>MKIVDVLCTPGLTGFYFDDQRAIKKGAGHDGFTYTGSTVTEGFTQVRQKGESISVLLVLEDGQVAHGDCAAVQYSGAGGRDPLFLAKDFIPVIEKEIAPKLIGREITNFKPMAEEFDKMTVNGNRLHTAIRYGITQAILDAVAKTRKVTMAEVIRDEYNPGAEINAVPVFAQSGDDRYDNVDKMIIKEADVLPHALINNVEEKLGLKGEKLLEYVKWLRDRIIKLRVREDYAPIFHIDVYGTIGAAFDVDIKAMADYIQTLAEAAKPFHLRIEGPMDVEDRQKQMEAMRDLRAELDGRGVDAELVADEWCNTVEDVKFFTDNKAGHMVQIKTPDLGGVNNIADAIMYCKANGMGAYCGGTCNETNRSAEVTTNIGMACGARQVLAKPGMGVDEGMMIVKNEMNRVLALVGRRK[2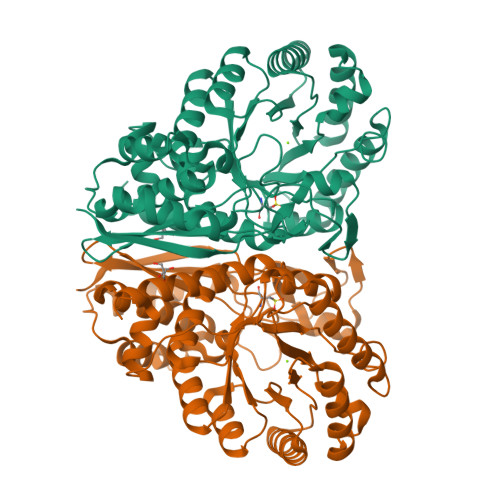x]> MAWPKVQPEVNIGVVGHVDHGKTTLVQAITGIWTSKHSEELKRGMTIKLGYAETNIGVCESCKKPEAYVTEPSCKSCGSDDEPKFLRRISFIDAPGHEVLMATMLSGAALMDGAILVVAANEPFPQPQTREHFVALGIIGVKNLIIVQNKVDVVSKEEALSQYRQIKQ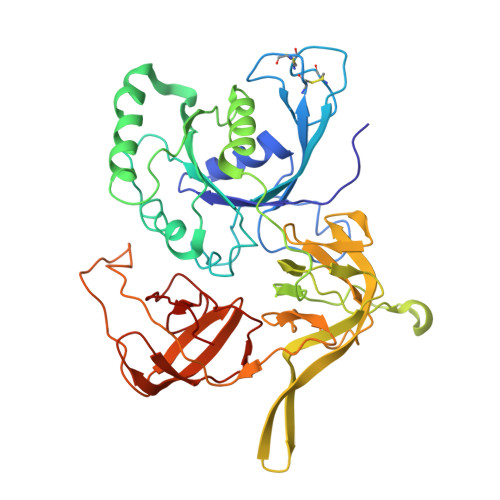FTKGTWAENVPIIPVSALHKINIDSLIEGIEEYIKTPYRDLSQKPVMLVIRSFDVNKPGTQFNELKGGVIGGSIIQGLFKVDQEIKVLPGLRVEKQGKVSYEPIFTKISSIRFGDEEFKEAKPGGLVAIGTYLDPSLTKADNLLGSIITLADAEVPVLWNIRIKYNLLERVVGAKEMLKVDPIRAKETLMLSVGSSTTLGIVTSVKKDEIEVELRRPVAVWSNNIRTVISRQIAGRWRMIGWGLVEI(1~{R})-1-cyclohexyl-2-[(5~{S})-6-fluoranyl-5~{H}-imidazo[1,5-b]isoindol-5-yl]ethanol | C18 H21 F 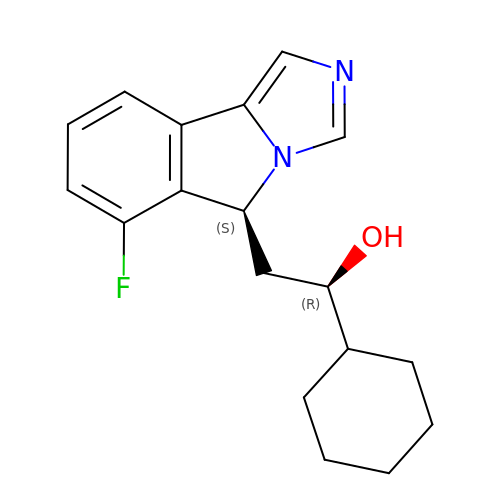N2 O | AKOIXTSNUPHRQM-DOTOQJQBSA-N> GKGGAKR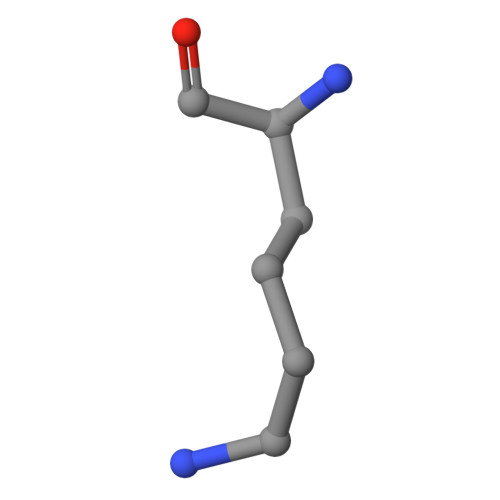HRKIL> MEMTSAFTLNVRLDNIAVITIDVPGEKMNTLKAEFASQVRAIIKQLRENKELRGVVFVSAKPDNFIAGADINMIGNCKTAQEAEALARQGQQLMAEIHALPIQVIAAIHGACLGGGLELALACHGRVCTDDPKTVLGLPEVQLGLLPGSGGTQRLPRLIGVSTALEMILTGKQLRAKQALKLGLVDDVVPHSILLEAAVELAKKERPSSRPLPVRERILAGPLGRALLFKMVGKKTEHKTQGNYPATERILEVVETGLAQGTSSGYDAEARAFGELAMTPQSQALRSIFFASTDVKKDPGSDAPPAPLNSVGILGGGLMGGGIAYVTACKAGIPVRIKDINPQGINHALKYSWDQLEGKVRRRHLKASERDKQLALISGTTDYRGFAHRDLIIEAVFENLELKQQMVAEVEQNCAAHTIFASNTSSLPIGDIAAHATRPEQVIGLHFFSPVEKMPLVEIIPHAGTSAQTIATTVKLAKKQGKTPIVVRDKAGFYVNRILAPYINEAIRMLTQGERVEHIDAALVKFGFPVGPIQLLDEVGIDTGTKIIPVLEAAYGERFSAPANVVSSILNDDRKGRKNGRGFYLYGQKGRKSKKQVDPAIYPLIGTQGQGRISAPQVAERCVMLMLNEAVRCVDEQVIRSVRDGDIGAVFGIGFPPFLGGPFRYIDSLGAGEVVAI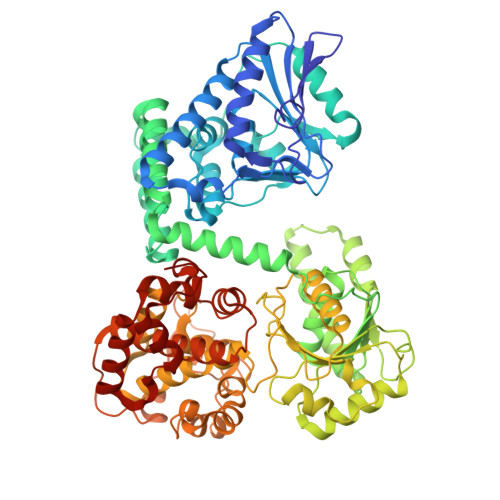MQRLATQYGSRFTPCERLVEMGARGESFWKTTA>GPGSMPWEVKADNAYGIDYNKLIDKFGCKLITKDMIERMERLTGQKAHHFFRRNIFLSHRDFEKILDVYEKGELFYLYTGRGPSSESLHVGHLVPFLFTKYLQDTFKVPLVIQLTDDEKFIFKSNLTLEETHNYAYENMKDIIACGFDPELTFIFTNLEYIAELYPDILRIEKKISCSQIKSIFGFKDSCNVGKFAFPAVQAAPAFSSSFPHIFGGRTDIHCLVPHAIDQDPYFRMVRDVAPRLGYLKPSSIHSIFLPSLQGSQTKMSASVQNSSIFVNDNEESIRNKIMKYAFSGGQATEEEQRRLGANLDVDVSWQYLRFLMEDDEKL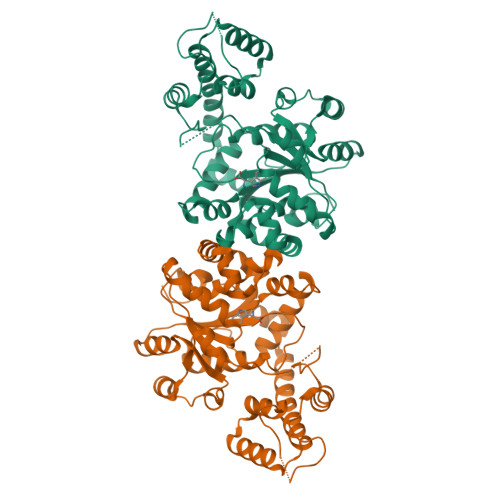EEIGKKYSSGEMLSGEIKSILVQELVKLTKNHQKNREAINDDVIAKFTNKSREQLLKLFINKK[2x]> MVGLTTLFWLGAIGMLVGTLAFAWAGRDAGSGERRYYVTLVGISGIAAVAYVVMALGVGWVPVAERTVFAPRYIDWILTTPLIVYFLGLLAGLDSRE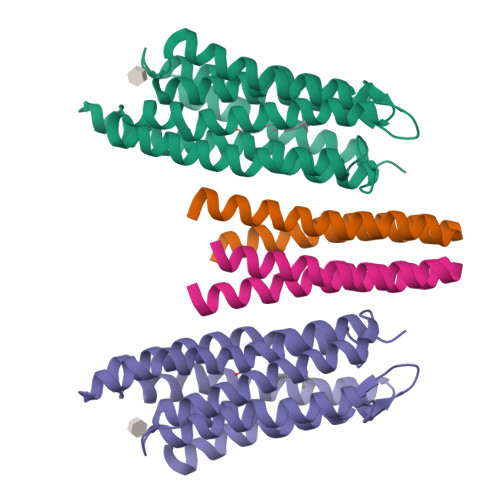FGIVITLNTVVMLAGFAGAMVPGIERYALFGMGAVAFLGLVYYLVGPMTESASQRSSGIKSLYVRLRNLTVILWAIYPFIWLLGPPGVALLTPTVDVALIVYLDLVTKVGFGFIALDAAATLRAEHGE;> GAVFIFVGALTVLFGAIAYGEVTAAAATGDAAAVQEAAVSAILGLIILLGINLGLVAATL>[2x]LTCVTSKSIFGITTENCPDGQNLCFKKWYYIVPRYSDITWGCAATCPKP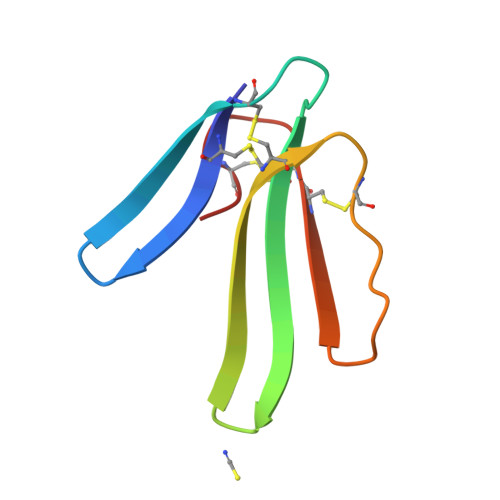TNVRETIRCCETDKCNE>MATPSMMPQWSYMHIAGQDASEYLSPGLVQFARATDTYFSLGNKFRNPTVAPTHDVTTDRSQRLTLRFVPVDREDTAYSYKVRFTLAVGDNRVLDMASTYFDIRGVLDRGPSFKPYSGTAYNSLAPKTAPNPCEWKDNNKIKVRGQAPFIGTNINKDNGIQIGTDTTNQPIYADKTYQPEPQVGQTQWNSEVGAAQKVAGRVLKDTTPMLPCYGSYAKPTNEKGGQASLITNGTDQTLTSDVNLQFFALPSTPNEPKAVLYAENVSIEAPDTHLVYKPDVAQGTISSADLLTQQAAPNRPNYIGFRDNFIGLMYYNSTGNMGVLAGQASQLNAVVDLQDRNTELSYQLMLDALGDRSRYFSMWNQAVDSYDPDVRIIENHGVEDELPNYCFPLGGSAATDTYSGIKANGQTWTADDNYADRGAEIESGNIFAMEINLAANLWRSFLYSNVALYLPDSYKITPDNITLPENKNTYAYMNGRVAVPSALDTYVNIGARWSPDPMDNVNPFNHHRNAGLRYRSMLLGNGRYVPFHIQVPQKFFAIKNLLLLPGSYTYEWNFRKDVNMILQSSLGNDLRVDGASVRFDSINLYANFFPMAHNTASTLEAMLRNDTNDQSFNDYLCAANMLYPIPSNATSVPISIPSRNWAAFRGWSFTRLKTKETPSLGSGFDPYFTYSGSVPYLDGTFYLNHTFKKVSIMFDSSVSWPGNDRLLTPNEFEIKRTVDGEGYNVAQCNMTKDWFLIQMLSHYNIGYQGFYVPESYKDRMYSFFRNFQPMSRQVVNTTTYKEYQNVTLPFQHNNSGFVGYMGPTMREGQAYPANYPYPLIGQTAVPSLTQKKFLCDRTMWRIPFSSNFMSMGALTDLGQNMLYANSAHALDMTFEVDPMDEPTLLYVLFEVFDVVRIHQPHRGVIEAVYLRTPFSAGNATT[12x];> MRRAVGVPPVMAYAEGPPPSYESVMGSADSPATLEALYVPPRYLGPTEGRNSIRYSELAPLYDTTRVYLVDNKSADIASLNYQNDHSNFQTTVVQNNDFTPAEAGTQTINFDERSRWGADLKTILRTNMPNINEFMSTNKFKARLMVEKKNKETGLPRYEWFEFTLPEGNYSETMTIDLMNNAIVDNYLEVGRQNGVLESDIGVKFDTRNFRLGWDPVTKLVMPGVYTNEAFHPDIVLLPGCGVDFTQSRLSNLLGIRKRLPFQEGFQIMYEDLEGGNIPALLDVAKYEASIQKAKEEGKEIGDDTFATRPQDLVIEPVAKDSKNRSYNLLPNDQNNTAYRSWFLAYNYGDPKKGVQSWTLLTTADVTCGSQQVYWSLPDMMQDPVTFRPSTQVSNYPVVGVELLPVHAKSFYNEQAVYSQLIRQSTALTHVFNRFPENQILVRPPAPTITTVSENVPALTDHGTLPLRSSISGVQRVTITDARRRTCPYVHKALGIVAPKVLSSRTF;> MQRSTAVVDGSQQVDPAMLAALQSQPSGVTPSDDWAAAMDRILALTTRNPEAFRQQPQANRFSAILEAVVPSRTNPTHEKVLAIVNALTESKAIRKDEAGLIYNALLERVARYNSTNVQANLDRLTTDVREAVAQRERFMHDTNLGSQVALNAFLSTLPANVPRGQEDYVSFISALRLLVAEVPQSEVYQSGPDYFFQTSRQGLQTVNLTQAFKNLQGMWGVRAPVGDRATISSLLTPNTRLLLLLIAPFTNSSTISRDSYLGHLITLYREAIGQTQVDEQTFQEITSVSRALG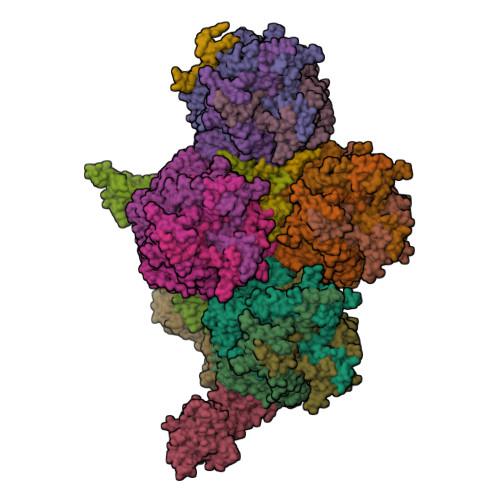QQDTGSLEATLNFLLTNRQQKIPSQFTLSTEEERILRYVQQSVSLYLMREGMTPSSALDMTARNMEPSLYSSNRPFINRLMDYLHRAAAMNSEYFTNAILNPHWMPPSGFYTGEFDMPEGDDGFLWDDVSDSIFVPARYRKKEGGDELPLPLVEAASRGQSPFPSLPSLVSSSNSGRVLRPRLPGETDYLNDPLLQPVRNKNFPNNGVESLVDKMNRWKTYAQEQREWEESQSRPLAGPFSRWRRREDDQDDSADDNSVLDLGGTGASSNPFAHLRPQGRLGRLY;>MSKEIPTPYMWSYQPQMGLAAGASQDYSSRMNWLSAGPHMIGRVNGIRATRNQILLEQAALTSTPRSQLNPPNWPAVQVYQENPAPTTVLLPRDAEAEVQMTNSGAQLAGGSRHVRFRGRSSPYSPGPIKRLIIRGRGIQLNDEVVSSLTGLRPDGVFQLGGAGRSSFTPRQAYLTLQSSSSQPRSGGIGTLQFVEEFVPSVYFNPFSGAPGLYPDDFIPNYDAVSESVDGYD[2x];>MSGSMEGNAVSFKGGVFSPYLTTRLPAWAGVRQNVMGSNVDGRPVAPANSATLTYATVGSSVDTAAAAAASAAASTARGMAADFGLYNQLAASRSLREEDALSVVLTRLEELSQQLQDLFAKVALLNPPANAS[4x];>MEDINFASLAPRHGSRPFMGTWNEIGTSQLNGGAFSWSSLWSGIKNFGSSIKSFGNKAWNSNTGQMLRDKLKDQNFQQKVVDGLASGINGVVDIANQALQNQINQRLENSRQPPVALKQRPTPEPEEVEVEEKLPPLETAPPLPSKGEKRPRPELEETLVVESREPPSYEQALKEGASYPMTRPIGSMARPVYGKEKTPVTLELPPPAPTVPPMPTPTLGTNVPRLAAPTVAVATPARRVRGANWQSTLNSIVGLGVKSLKRRRCY[4x];>[2x]MSILISPDNNTGWGLHSAGMYGGAKRRSSQHPVRVRGHYRAPWGAHTRGIISGRTTVDDVIDSVVADARRYQRPTSTVDSVIDSVVADARRYAQRKSRLRRRRRRPTTAMIAARAVLRRARRIGRRAMRRAAAAASAGRARRQAARQAAAAIASMAQPRRGNVYWVRDASGVRVPVRTRPPRS>SNAMAEKLLHTAESDAGIGSWVLHMESGRLEWSQAVHDIFGTDSATFDATEDAYFQRVHPDDRARVRRELDRHVLGDRPFDVEYRIVRP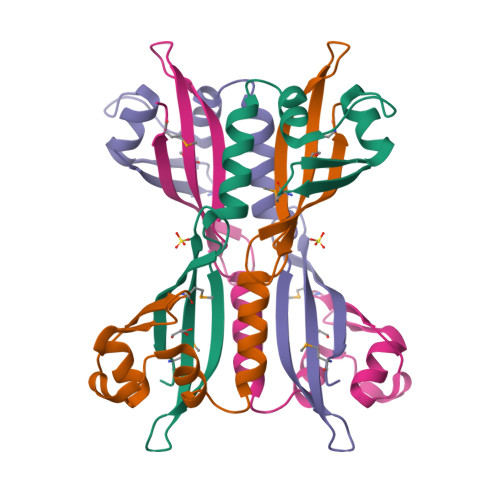DGQVRELLERNHIQRQASGQVDHLWGTVIDMTEHKQ[4x]(2S)-2-AMINO-5-(2-(METHYLSULFINYL)ACETIMIDAMIDO)PENTANOIC 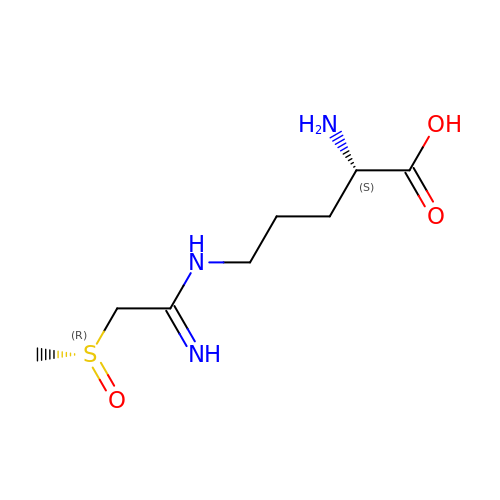ACID | C8 H17 N3 O3 S | PZGMBMRDRVWIGU-WDDATRMLSA-N> 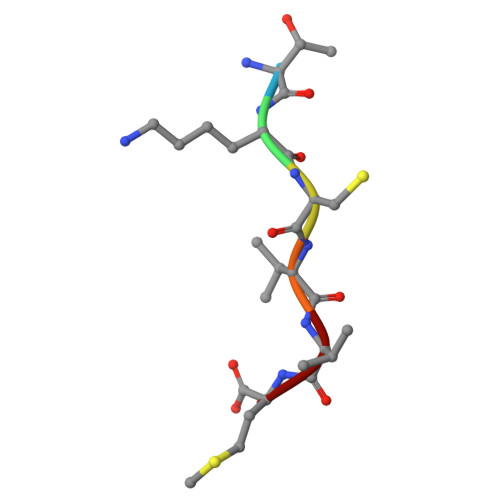TKCVVM> LSKYGGECSKKDNTCTYRKDGKDHIVKCPSADNKKCKTDRHHCEYDDHHKTVDCQ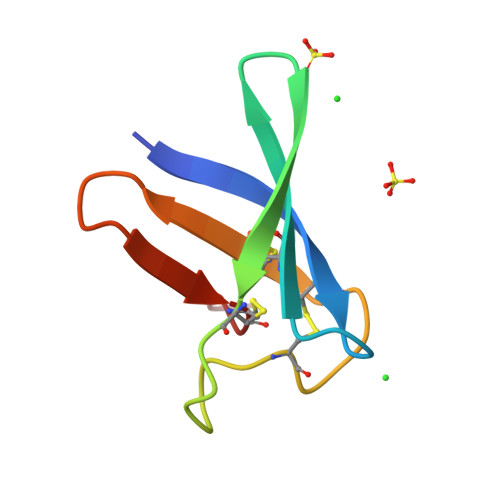TPV> MLKHIISAYNFSRDELEDIFALTD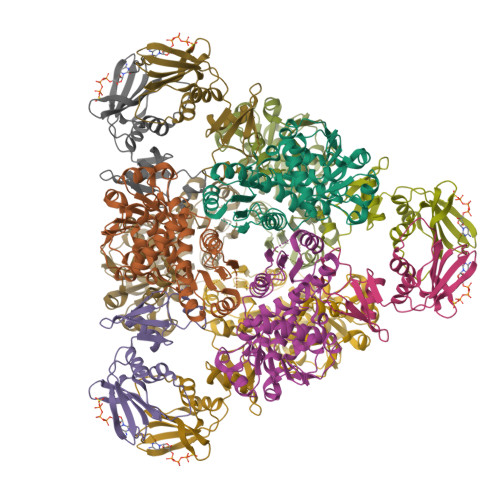KYSKNLNDTRKILSGKTISIAFFEPSTRTYLSFQKAIINLGGDVIGFSGEESTSVAKGENLADTIRMLNNYSDGIVMRHKYDGASRFASEISDIPVINAGDGKHEHPTQAVIDIYTINKHFNTIDGLVFALLGDLKYARTVNSLLRILTRFRPKLVYLISPQLLRARKEILDELNYPVKEVENPFEVINEVDVLYVTRIQKERFVDEMEYEKIKGSYIVSLDLANKMKKDSIILHPLPRVNEIDRKVDKTTKAKYFEQASYGVPVRMSILTKIYGE;> MEFMMEIQGNRKELMVSKIKNGTVIDHIPAGRAFAVLNVLGIKGHEGFRIALVINVDSKKMGKKDIVKIEDKEISDTEANLITLIAPTATINIVREYEVVKKTKLEVPKVVKGILKCPNPYCITSNDVEAIPTFKTLTEKPLKMRCEYCETIIDENEIMSQILGANNK> ELTPDQATLLHFIMDSYNKQRMPQEITNKILKEAFSAEENFLILTEMATNHVQVLVE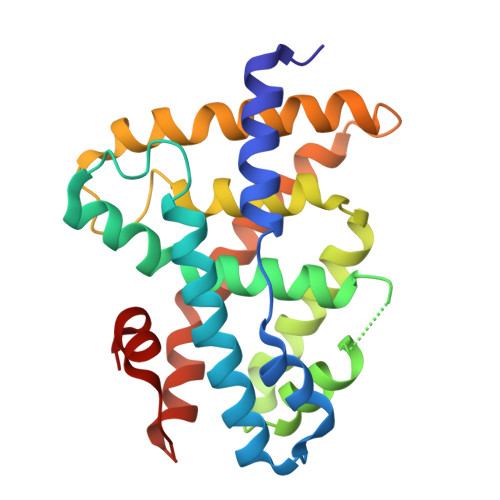FTKKLPGFQTLDHEDQIALLKGSAVEAMFLRSAEIFNKKLPSGHSDLLEARIRNSGISDEYITPMFSFYKSIGELKMTQEEYALLTAIVILSPDRQYIKDREAVEKLQEPLLDVLQKLCKIHQPANPQHFAKLLGRLTELRTFNHHHAEMLMSWRVNDHKFTPLLQEIWDV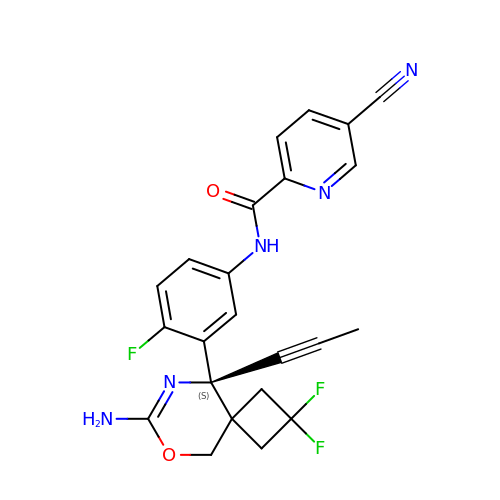N-[3-[(9S)-7-azanyl-2,2-bis(fluoranyl)-9-prop-1-ynyl-6-oxa-8-azaspiro[3.5]non-7-en-9-yl]-4-fluoranyl-phenyl]-5-cyano-pyridine-2-carboxamide | C23 H18 F3 N5 O2 | GBDJTQDCHCBNSY-HSZRJFAPSA-N>PVPRSCAEPAGIPALLSPRDKLAQLLVVGVRDAADAQAVVTNYHVGGILIGSDTDLTIFDGALAEIVAGGGPLPLAVSVDEEGGRVSRLRSLIGGTGPSARELAQTRTVQQVRDLARDRGRQMRKLGITIDFAPVVDVTDAPDDTVIGDRSFGSDPATVTAYAGAYAQGLRDAGVLPVLKHFPGHGRGSGDSHNGGVTTPPLDDLVGDDLVPYRTLVTQAPVGVMVGHLQVPGLTGSEPASLSKAAVNLLRTGTGYGAPPFDGPVFSDDLSGMAAISDRFGVSEAVLRTLQAGADIALWVTTKEVPAVLDRLEQALRAGELPMSAVDRSVVRVATMKG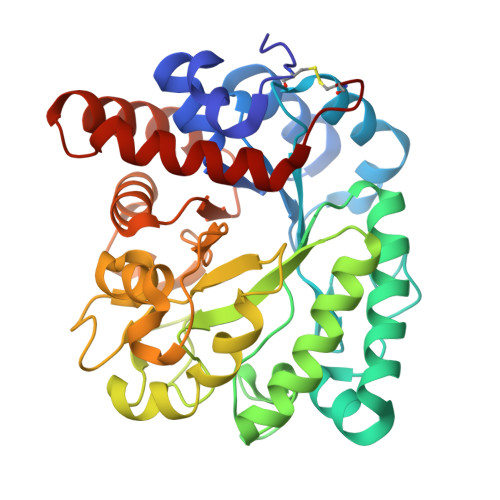PNPGC[2x]> GMASLKAKVLETFLAKSRPELLEYYIKVILDYNTAHNKVALSECYTVASVAEMPQNYRPHPQRFTYCSQVLGLHCYKKGIHYWEVELQKNNFCGVGICYGSMNRQGP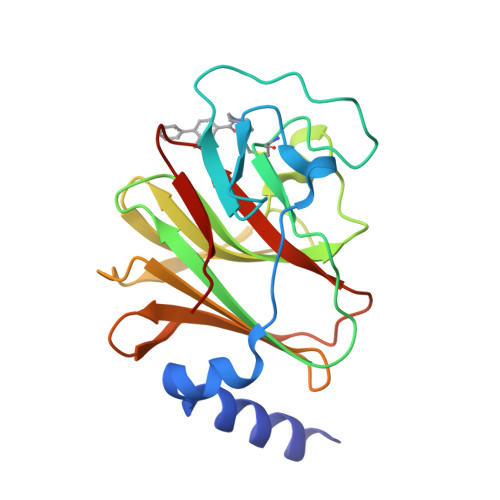ESRLGRNSASWCVEWFNTKISAWHNNVEKTLPSTKATRVGVLLNCDHGFVIFFAVADKVHLMYKFRVDFTEALYPAFWVFSAGATLSICSPK>[2x]MISSQQAMVHVVS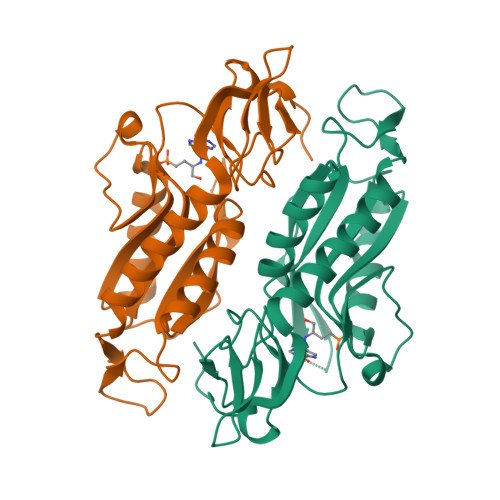RNAEGVIVVDGKAYPMAEELVATESVIQRSIKAVAKQIADFYRPLSHRDTHGGGGVAPISDENPLIIISVLKGSYIFTADMVRYLGDYGLPHVVDFLRVASYRGTSSTNKMQLLAETQFKALRGKHVLILEDIVDSGKTLRYILDKVQREHQPATLKVCVLADKPGGRRVTMQPDFVCLTVPNKYVIGYGFEVNDRFRCFRHIFTLRPGEARRYPAHL> AVNRLQHHHHHHHLEGTVTTDGADIVIKTKGGLEVATTDKEFSFKLGGRLQADYSRFDGFYTKNGNTADAAYFRRAFIELGGTAYKDWKYQINFDLSHNTGSSDNGYFDEASVTYTGFNPVNLKFGRFDPDFGLEKATSSKWVTAPERNAAYELADWINTHQDGMGAQVNSTLADMAYLSAGVSAKDADDSDGDSVKQFNFRGVFAPMHEAGNVLHVGVNYAYRDLDDTAFDSRIRPRLGMRGIATSGGNDAGDNGNRATFGGVSNSPAGSYKDDSVWGLEGAWAMGPFSAQAEYLARKLKADDNAYKDIKAKGYYAQLAYTLTGESRQYKLEGAKFDSVKPENKEIGAWEVFYRYDNIKVEDDNVVADTATREV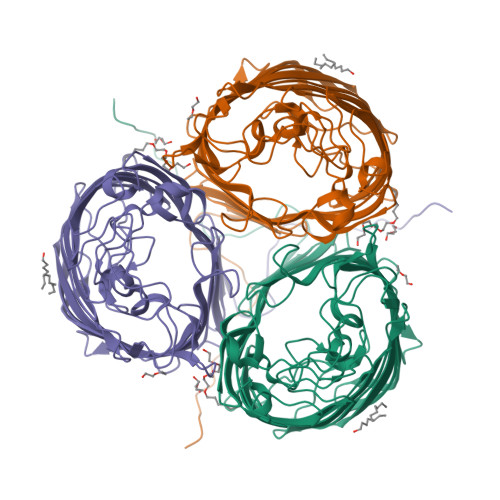GDTKAKAHNLGVNWYVNDAVKISAAYVKAKTDKITNNNGDDDGDGFVTRLQYVF>[4x]MNVAPKFLANMTSVILPEDLPVGAQAFWLVAEDQDNDPLTYGMSGPNAYFFAVTPKTGEVKLASALDYETLYTFKVT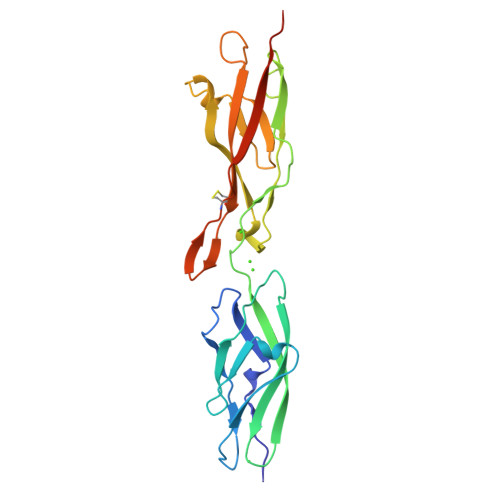ISVSDPYIQVQREMLVIVEDRNDNAPVFQNTAFSTSINETLPVGSVVFSVLAVDKDMGSAGMVVYSIEKVIPSTGDSEHLFRILANGSIVLNGSLSYNNKSAFYQLELKACDLGGMYHNTFTIQCSLPVFLSISVVDQPDLEHHHHHH> MGSWSHPQFEKGSSKATEQNDKLKRAIIISAVLHVILFAALIWSSFDENIEASAGGGGGSSIDAVMVDSGAVVEQYKRMQSQESSAKRSDEQRKMKEQQAAEELREKQAAEQERLKQLEKERLAAQEQKKQAEEAAKQAELKQKQAEEAAAKAAADAKAKAEADAKAAEEAAKKAAADAKKKAEAEAAKAAAEAQKKAEAAAAALKKKAEAAEAAAAEARKKAATEAAEKAKAEAEKKAAAEKAAADKKAAAEKAAADKKAAEKAAAEK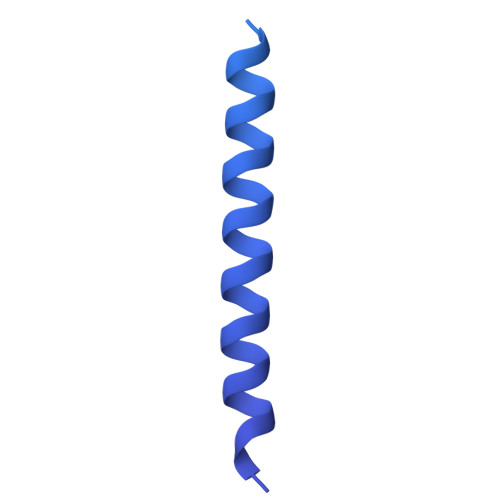AAADKKAAAEKAAADKKAAAAKAAAEKAAAAKAAAEADDIFGELSSGKNAPKTGGGAKGNNASPAGSGNTKNNGASGADINNYAGQIKSAIESKFYDASSYAGKTCTLRIKLAPDGMLLDIKPEGGDPALCQAALAAAKLAKIPKPPSQAVYEVFKNAPLDFKP> SMDCRTKANPDRTFDLVLKVKCHASENEDPVVLWKFPEDFGDQEILQSVPKFCFPFDVERVSQNQVGQHFTFVLTDIESKQRFGFCRLTSGGTICLCILSYLPWFEVYYKLLNTLADYLAKELENDLNETLRSLYNHPVPKANTPVNLSVHSYFIAPDVTGLPTIPESRNLTEYFVAVDVNNMLQLYASMLHERRIVIISSKLSTLTACIHGSAALLYPMYWQHIYIPVLPPHLLDYCCAPMPYLIGIHSSLIERVKNKSLEDVVMLNVDTNTLESPFSDLNNLPSDVVSALKNKLKKQSTATGDGVARAFLRAQAALFGSYRDALRYKPGEPITFCEESFVKHRSS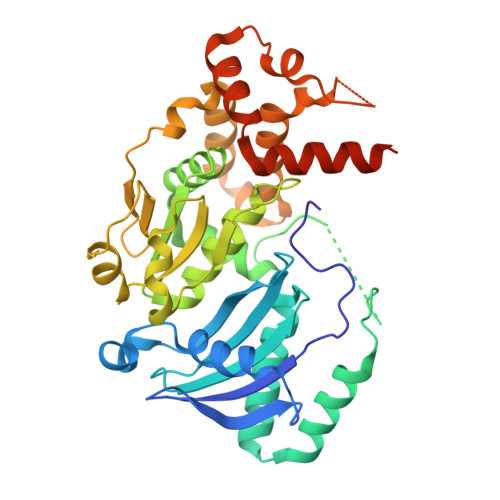VMKQFLETAINLQLFKQFIDGRLAKLNAGRGFSDVFEEEITSGG> MGHHHHHHLYFQGMNRPSFNEAWLAFRKVNHSVADVGSIIGGNVGKNITGGYFQNACPIRMSYVLNATGFPIARNSPYAKVSGADNKFYIYRVNDMIDYLTHTMGKPDLIVNNPKQSDFIGKKGIIVVKGHGWSNARGHVTLWNGSICSDQCHLLNDPDNGPFVPEVGTLWILP;> QEALTTQYSQSELLKNWALSHCLALVYKDDVVKNDARATASAYLEYGKQSVEIYHEIDEIAKKYSGLKYNGSISSDFNTMKCIDFIHDRELNELIKRRVEK

We therefore determined the three-dimensional structure of the Tae4/Tai4 effector/immunity system from Salmonella typhimurium by X-ray crystallography. Tae4 cleaves the γ-D-glutamyl-L-meso-diaminopimelic acid amide bond as do Tae1 members; however, it specifically hydrolyzes the acceptor stem of the muropeptides. Thus, Tae4 adopts the classical papain-like fold of cysteine peptidases of the NlpC/P60 family. Moreover, the immunity protein Tai4 represents a new family of T6SS immunity proteins forming a heterotetramer with its cognate effector Tae4.

Crystals of the effector/immunity system Tae4/Tai4 from S. typhimurium readily grew to a size of 400×100×100 µm3 within 3 days in 2-ethoxyethanol containing conditions. Experimental phases were obtained from a Single-wavelength Anomalous Diffraction (SAD) experiment and an initial structure was built and refined to a resolution of 2.3 Å. Native protein crystals of identical crystal symmetry diffracted to a resolution of 1.8 Å at the Swiss Light Source (Villigen, CH), allowing the refinement of a structural model at near atomic resolution. Both models were finally refined to excellent stereochemistry, with 97% of the residues in preferred regions of the Ramachandran plot. The core of the Tae4 effector is formed by a central antiparallel β-sheet flanked by α-helices. As a true NlpC/P60 papain-like cysteine peptidase, Tae4 has a catalytically important cysteine residue (Cys44) in its active site. Similar to Tsi1, Tae4 locks up the active site by inserting the loop region between the α-helices d and e (d-e-loop) into the active site and thereby prevents substrate binding and catalysis. Most importantly, the hydroxyl group of Ser98 in this loop forms a hydrogen bond to the Nδ atom of the catalytic His126 of Tae4, preventing it from deprotonating the catalytic Cys44 residue. In contrast to the Tse1/Tsi1 complex which has been reported to be a heterodimer, we found that the inhibited Tae4/Tai4 protein complex from S. typhimurium forms heterotetramers. In this heterotetrameric assembly, the two polypeptide chains of a Tai4 homodimer inhibit two Tae4 molecules.The Streptococcus pneumoniae gene SP_1669 encodes a Nudix hydrolase. The gene is located in an operon containing MurF, suggesting that it plays a role in the Mur pathway of peptidoglycan biosynthesis by hydrolyzing Mur pathway substrates. This enzyme contains a modified Nudix signature sequence, GX5YX7KEUXEEXGU, in which a conserved glutamate/arginine pair that forms a hydrogen bond in the canonical motif is substituted by a tyrosine/lysine pair (position 7 and 13 of the signature sequence). The enzyme robustly hydrolyzes these compounds, indicating that it is a UDP-X diphosphatase (UDP-Xase) that hydrolyzes substrates of the form of UDP linked to some moiety X (UDP-X). The UDP-Xase from Streptococcus pneumoniae, may be a member of a novel Nudix hydrolase family whose members fold as asymmetric homodimers and act on bacterial cell wall precursors as well as RNA.

The 1.39 Å resolution structure of this enzyme shows that it is an asymmetric homodimer with two distinct catalytic sites, one “open” and one “closed-in”. The C-terminal catalytic domain contains the Nudix signature sequence that encodes residues involved in Mg2+ binding and catalysis. The two C-terminal catalytic domains form a symmetric dimer stabilized by an extensive network of salt bridges and hydrogen bonds formed by Gln200, Leu127, Asp203, Thr107, Phe146, Gly103, Tyr104, Asp132, and Gln142. The two HLH motifs stack against each other to form a four-helix bundle. The approximate two-fold axis of symmetry relating the N-terminal HLH motifs does not coincide with the two-fold axis of the C-terminal catalytic domain dimer, making UDP-Xase an asymmetric homodimer. The asymmetric dimer has two different Nudix active sites, each with the conserved Nudix box sequence. The “closed-in” site can accommodate a Nudix substrate but is too small to engage RNA. However, although the “open” site could potentially bind Nudix substrates, its cavity is large enough to accommodate an RNA molecule. The “closed-in” site, formed by the N- terminal domain of monomer A and the C-terminal domain of monomer B of the UDP-Xase dimer, is ideally suited for binding UDP-N-acetylmuramoyl-L-alanine and possibly longer Mur pathway substrates such as UDP-N-acetylmuramoyl-L-alanine-D-glutamate-L-lysine.

>MKTSDFVKYLQRMIAITDTGLTFTKDPFDRERYEDLRSLLSEMLNQASDLDSEEVAEVLKPTSAYATPLMDVRAWIVEDEKICLVRGQGEDSWALPGGFGEVGYSPTENILKEIEEETGFKAKVERLLAVFDTNRFQLQSKQYTKFVFGCKLLDGQFQENQEIADLQFFAIDQLPNLSEKRITKEQIELLWQVYQGHRGQYLD[2x]> MTWPVKDFNYSDPVNDNDILYLRIPQNKLITTPVKAFMITQNIWVIPERFSSDTNPSLSKPPRPTSKYQSYYDPSYLSTDEQKDTFLKGIIKLFKRINERDIGKKLINYLVVGSPFMGDSSTPEDTFDFTRHTTNIAVEKFENGSWKVTNIITPSVLIFGPLPNILDYTASLTLQGQQSNPSFEGFGTLSILKVAPEFLLTFSDVTSNQSSAVLGKSIFCMDPVIALMHQLTYSLHQLYGINIPSDKRIRPQVSEGFFSQDGPNVQFEELYTFGGLDVEIIPQIERSQLREKALGHYK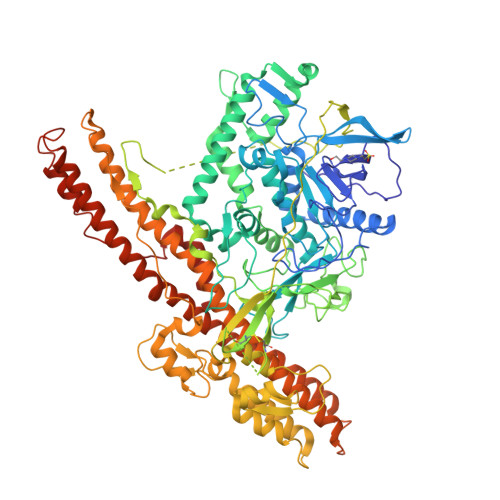DIAKRLNNINKTIPSSWISNIDKYKKIFSEKYNFDKDNTGNFVVNIDKFNSLYSDLTNVMSEVVYSSQYNVKNRTHYFSRHYLPVFANILDDNIYTIRDGFNLTNKGFNIENSGQNIERNPALQKLSSESVVDLFTKVCVDKSEEKLYDDDDKDRWGSSLQCIKVKNNRLPYVADKDSISQEIFENKIITDETNVQNYSDKFSLDESILDGQVPINPEIVDPLLPNVNMEPLNLPGEEIVFYDDITKYVDYLNSYYYLESQKLSNNVENITLTTSVEEALGYSNKIYTFLPSLAEKVNKGVQAGLFLNWANEVVEDFTTNIMKKDTLDKISDVSVIIPYIGPALNIGNSALRGNFNQAFATAGVAFLLEGFPEFTIPALGVFTFYSSIQEREKIIKTIENCLEQRVKRWKDSYQWMVSNWLSRITTQFNHINYQMYDSLSYQADAIKAKIDLEYKKYSGSDKENIKSQVENLKNSLDVKISEAMNNINKFIRECSVTYLFKNMLPKVIDELNKFDLRTKTELINLIDSHNIILVGEVDRLKAKVNESFENTMPFNIFSYTNNSLLKDIINEYFNLEAHHHHHHHHHH>GEVINQPMMMAARQLHDEARKWSSKGNDIIAAAKRMALLMAEMSRLVRGGSGTKRALIQCAKDIAKASDEVTRLAKEVAKQCTDKRIRTNLLQVCERIPTISTQLKILSTVKATMLGRTNISDEESEQATEMLVHNAQNLMQSVKETVREA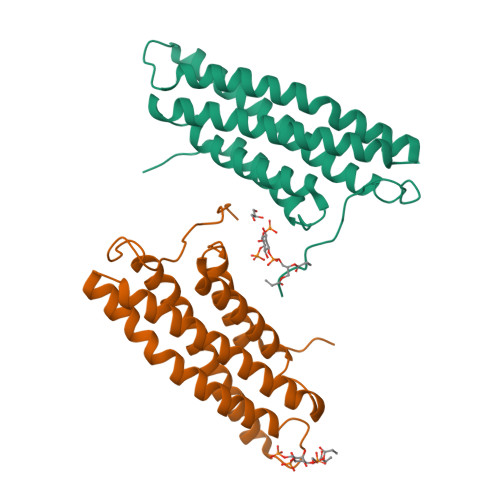EAASIKIRTDAGFTLRWVAKTPWYQ[6x]>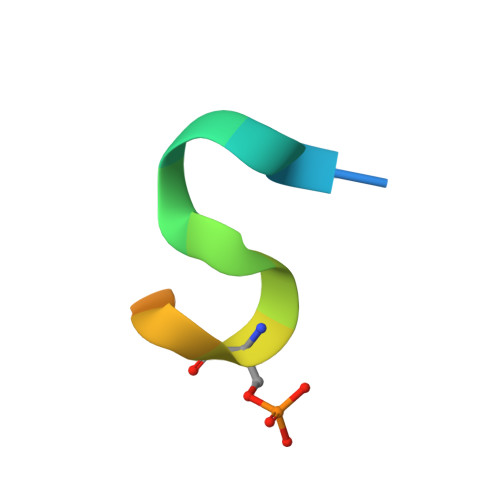 MEELLNLCSGKFTSQD(3S)-pyrazolidin-3-amine | C3 H9 N3 | 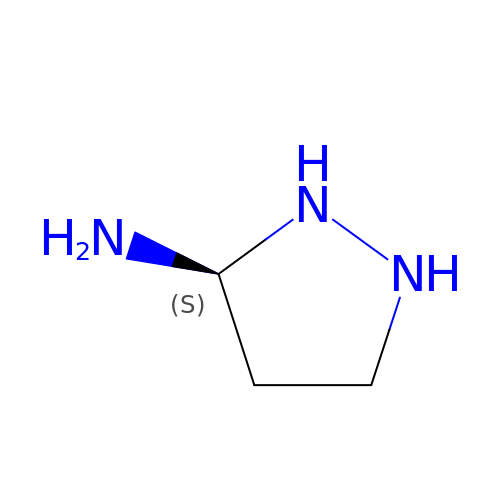LVMKSXJAVMOGQR-VKHMYHEASA-N>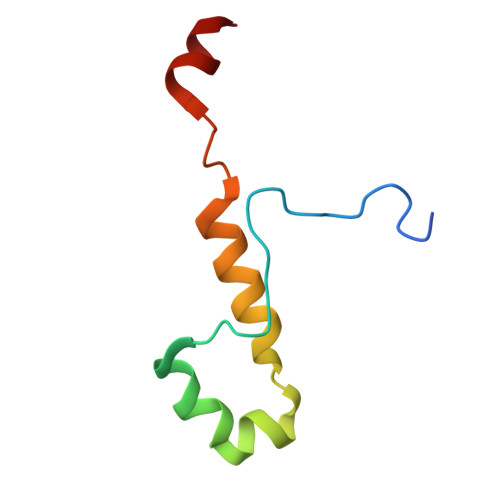 GPYDPFGGMEFVPSRYRVREELNHPSLDKYRIDQQHITGGYSFLDYISRAMFEAFAGLAVFIEDEKEAG>[2x]GAMPHDPSFTPTQ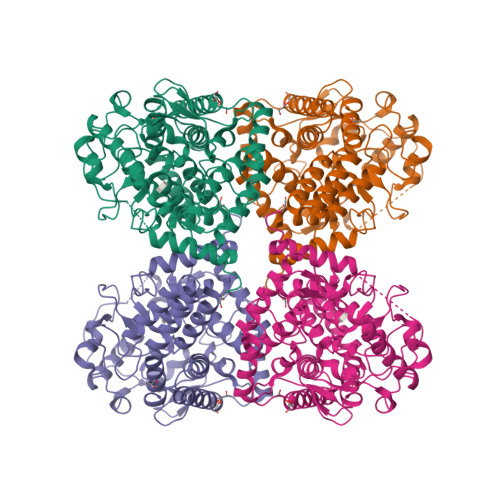LAARAAYLLRGNDLGTMTTAAPLLYPHMWSWDAAFVAIGLAPLSVERAVVELDTLLSAQWRNGMIPHIVFANGVDGYFPGPARWATATLADNAPRNRLTSGITQPPVHAIAVQRILEHARTRGRSTRAVAEAFLDRRWGDLMRWHRWLAECRDRNERGRITLYHGWESGMDNSPRWDSAYANVVPGKLPEYQRADNVIITDPSQRPSDGEYDRYLWLLEEMKAVRYDDERLPSVMSFQVEDVFFSAIFSVACQVLAEIGEDYKRPHADVKDLYLWAERFRAGVVETTDQRTGAARDFDVLAEKWLVTETAAQFAPLLCGGLPHDRERALLKLLEGPRFCGHPDLKYGLIPSTSPVSRDFRPREYWRGPVWPVLTWLFSWCFARRGWAERARLLRQEGLRQASDGSFAAYYEPFTGEPLGSMQQSWTAAAVLDWLG>MRVILFDLDGTLIDSAKDIALALEKTLKELGLEEYYPDNVTKYIGGGVRALLEKVLKDKFREEYVEVFRKHYLENPVVYTKPYPEIPYTLEALKSKGFKLAVVSNKLEELSKKILDILNLSGYFDLIVGGDTFGEKKPSPTPVLKTLEILGEEPEKALIVGDTDADIEAGKRAGTKTALALWG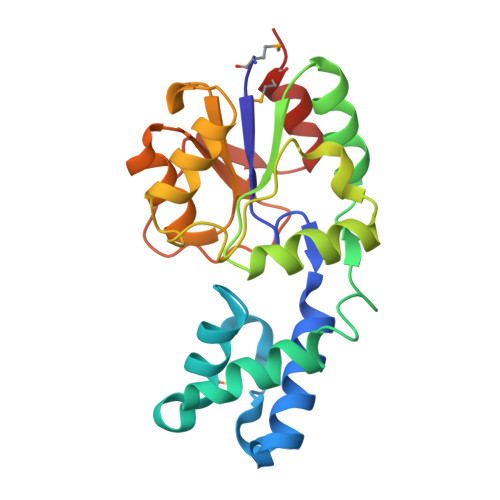YVKLNSQIPDFTLSRPSDLVKLMDNHIVEF[2x]>[2x]WQNSYLGKFLCVPNLEGRWHVDGHTRSEGG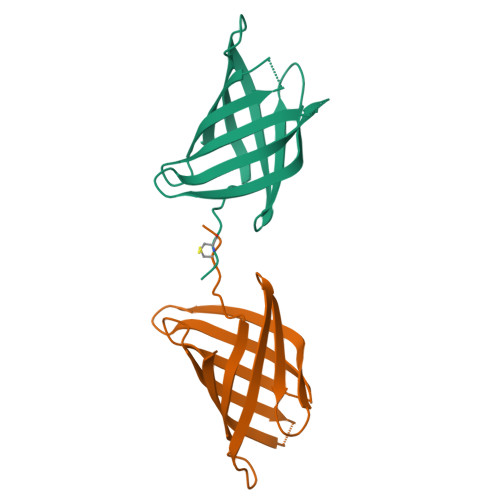NTWEGELKIVQTWDKVRIHLKTKASHSDSVTASIIYDKGIGYQLLYNYRNQPKTGEEHLTSHVGFAEFRFDADLKSAEGHYFNGQGRATYGTMTITRIEHA> MATNNNQIGENKEQTI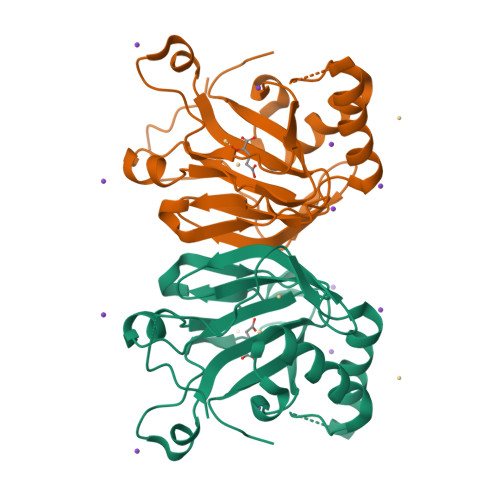FDHKGNVIKTEDREIQIISKFEEPLIVVLGNVLSDEECDELIELSKSKLARSKVGSSRDVNDIRTSSGAFLDDNELTAKIEKRISSIMNVPASHGEGLHILNYEVDQQYKAHYDYFAEHSRSAANNRISTLVMYLNDVEEGGETFFPKLNLSVHPRKGMAVYFEYFYQDQSLNELTLHGGAPVTKGEKWIATQWVRRGTYK> MQMSPALTCLVLGLALVFGEGSAVHHPPSYVAHLASDFGVRVFQQVAQASKDRNVVFSPYGVASVLAMLQLTTGGETQQQIQAAMGFKIDDKGMAPALRHLYKELMGPWNKDEISTTDAIFVQRDLKLVQGFMPHFFRLFRSTVKQVDFSEVERARFIINDWVKTHTKGMISNLLGKGAVDQLTRLVLVNALYFNGQWKTPFPDSSTHRRLFHKSDGSTVSVPMMAQTNKFNYTEFTTPDGHYYDILELPYHGDTLSMFIAAPYEKEVPLSALTNILSAQLISHWKGNMTRLPRLLVLPKFSLETEVDLRKPLENLGMTDMFRQFQADFTSLSDQEPLHVAQALQKVKIEVNESGTVASSSTAVIVSARMA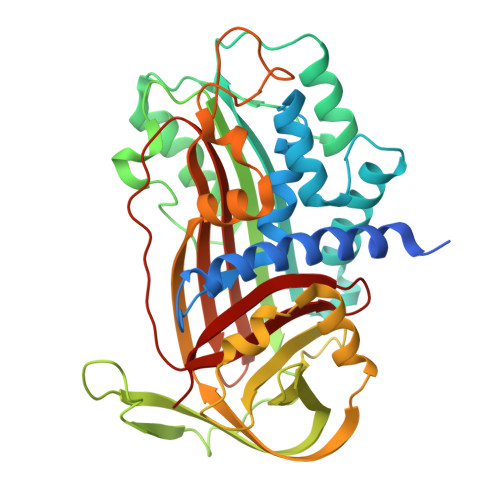PEEIIMDRPFLFVVRHNPTGTVLFMGQVMEP>[2x]MGALARALLLPLLAQWLLRAAPELAPAPFTLPLRVAAATNRVVAPTPGPGTPAERHADGLALALEPALASPAGAANFLAMVDNLQGDSGRGYYLEMLIGTPPQKLQILVDTGSSNFAVAGTPHSYIDTYFDTERSSTYRSKGFDVTVKYTQGSWTGFVGEDLVTIPKGFNTSFLVNIATIFESENFFLPGIKWNGIL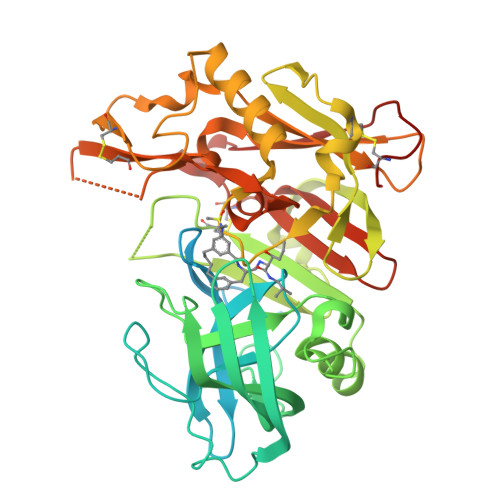GLAYATLAKPSSSLETFFDSLVTQANIPNVFSMQMCGAGLPVAGSGTNGGSLVLGGIEPSLYKGDIWYTPIKEEWYYQIEILKLEIGGQSLNLDCREYNADKAIVDSGTTLLRLPQKVFDAVVEAVARASLIPAFSDGFWTGSQLACWTNSETPWSYFPKISIYLRDENSSRSFRITILPQLYIQPMMGAGLNYECYRFGISPSTNALVIGATVMEGFYVIFDRAQKRVGFAASPCAEIAGAAVSEISGPFSTEDVASNCVPA>[4x]MTETVHKLDTNSTSQDDYVNQEELNYLNQLKDIIDHGVRKNDRTGIGTLSTFGTQSRYCLRDDIFPLLTTKRVFWRGVVEELLWFISGSTNAKQLSEKNVNIWDGNSSREFLDSRGLYNYEEGDLGPVYGFQWRHFGCPYSSMTADYKGKGYDQL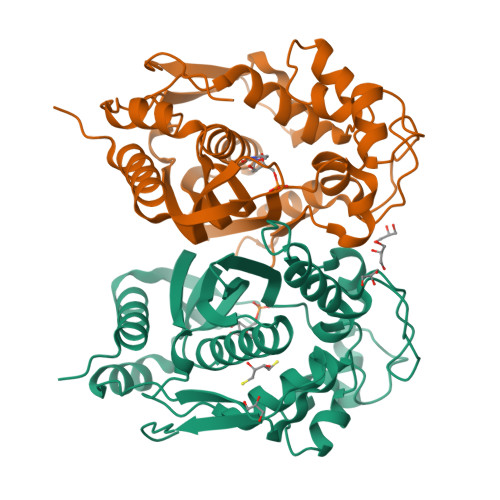QQCIKMIREEPESRRIIMTAWNPCDLEKVALPPCHCFVQFYVADGELSCQMYQRSADMGLGVPFNIASYSLLTRMIAHITSLKPGFFIHTIGDAHVYLTHVDALKVQMERKPRPFPKLKILRNVENIDDFRAEDFELINYKPYPKISMPMAV> MWVDFIDQTKSLKVSVNNYFYYLDRIKKLFTYLNDLRKHILKKYVYTINHKRIAINYLYFSMVTGLSGAALATMIRLELAHPGSPFFKGDSLRYLQVVTAHGLIMVFFVVVPILFGGFANFLIPYHVGSKDVAYPRLNSIGFWIQPCGYILLAKIGFLRPQFWRYYDKTSFSFPFLEKMKYNQYKEYKNDYLFYLDFLKKEITDDHSFFWKARKVIKLPQYSVFSFVPLKLMMWKTMINYPESFWYAASRVVQSRRKKVFVTKCSARTLTTAGWTFITPFSSNIKYTAVGSQDILILSVVFAGISTTISFTNLLITR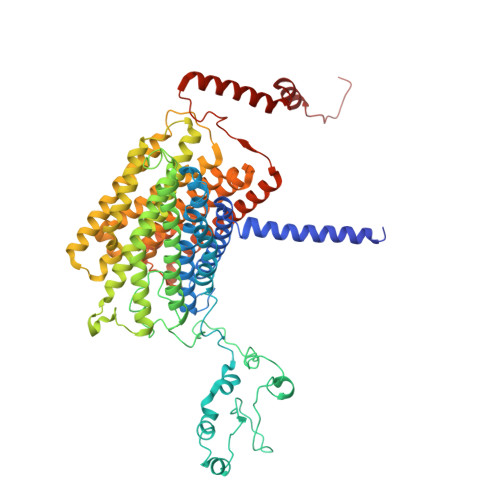RTLAMPGLRHRRVLMPFVTISIFLTLRMLATITPVLGAAVIMMAFDRHWQTTFFEYAYGGDPILSQHLFWFFGHPEVYVLIIPTFGFINMIVPHNNTRRVASKHHMIWAIYVMAYMGYLVWGHHMYLVGLDHRSRTMYSTITIMISMPATIKVVNWTLSLVNGALKIDLPFLFSMSFLLLFLVAGFTGMWLSHVSLNVSMHDTFYVVAHFHIMLSGAAMTGIFSGIYYYFNALFGVKYSRMFGYMHLIYYSGGQWVAFVPLFYLGFSGMPRRIHDYPVVFMGWHSMSTTGHFITLVGIIFFFLMMFDSHIERRASTSTTLGLPRWYKRISYYIFKIRYLQHTKSKMNGIPGSTVRLMLINRHFVEYEVYEK>[2x]MLCDSLPTASRTAAAILNLAQSEDVTAEALAQLIQTDPALTGRILRFANAPAQGTRRPVASVIDAIDLVGLPAVRQFALSLSLIDAHREGRCEAFDYAAYWQKSLARAVALQSITAQASTVAPKEAFTLGLLADV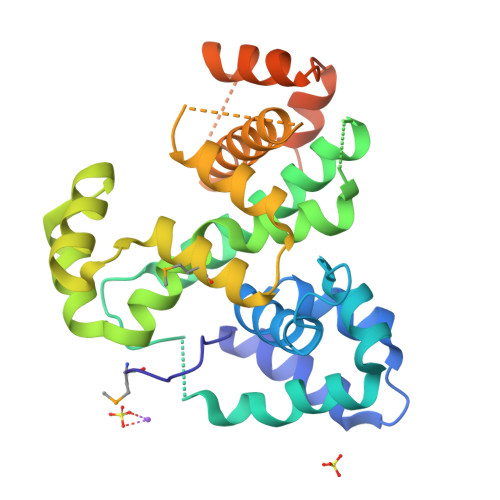GRLALATAWPEEYSECLRKADGEALIALERERFATDHDELTRMLLTDWGFPQVFIDALQLSQQDEIRDEGRTGRFARQLTLAQHIADHRLAEEPRRAALSPLLRAEARRCGLGDEDLARLLADPPADWLDRTRTIGLGGDLEHHHHHH N-acetyl-D-glucosamine-6-phosphate 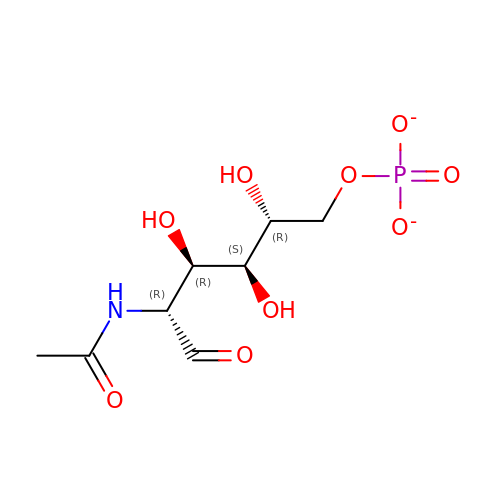| C8 H14 N O9 P | QDSLHWJDSQGPEE-LXGUWJNJSA-L>[2x]MELRVGNRYRLGRKIGSGSFGDIYLGTDIAAGEEVAIKLECVKTKHPQLHIESKIYKMMQG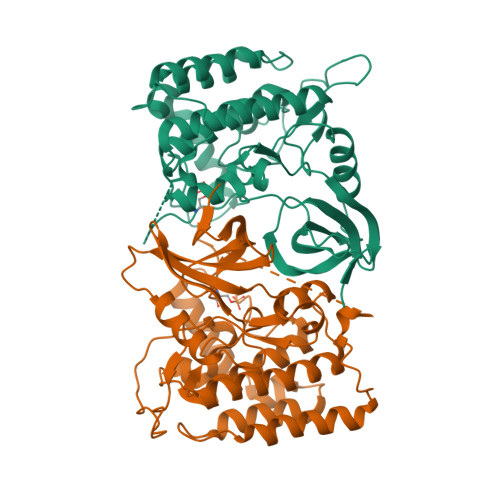GVGIPTIRWCGAEGDYNVMVMELLGPSLEDLFNFCSRKFSLKTVLLLADQMISRIEYIHSKNFIHRDVKPDNFLMGLGKKGNLVYIIDFGLAKKYRDARTHQHIPYRENKNLTGTARYASINTHLGIEQSRRDDLESLGYVLMYFNLGSLPWQGLKAATKRQKYERISEKKMSTPIEVLCKGYPSEFATYLNFCRSLRFDDKPDYSYLRQLFRNLFHRQGFSYDYVFDWNMLKQDTSRMSTSQIPGRVASSGLQSVVHR>[4x]MRVAIPAEDDRGIKSNVSKHFGRSRYFVFVDIEGEDVKNVEVVEVPFEEHGPGDLPNF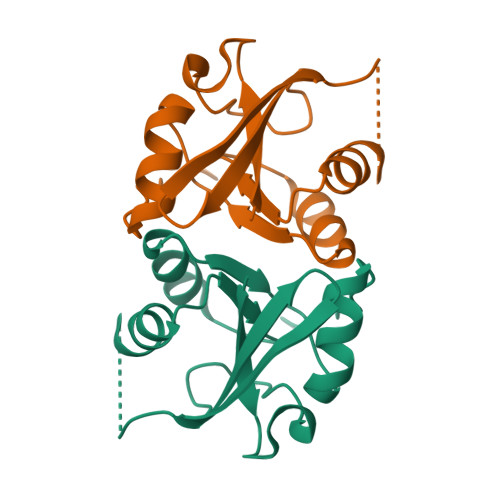IKDHGAKIVLTYGIGRRAIEYFNSLGISVVTGVYGRISDVIKAFIGGKLKIDYDWKEKIEKEH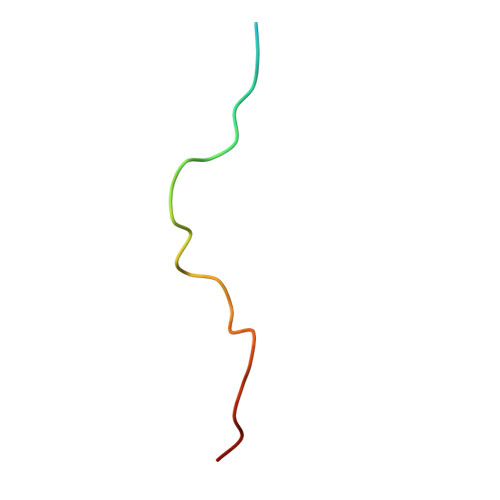> SRRRRRRKRKREWDDDDDPPKKRRRLD>[2x]MLSPELLAKAFPFHFAF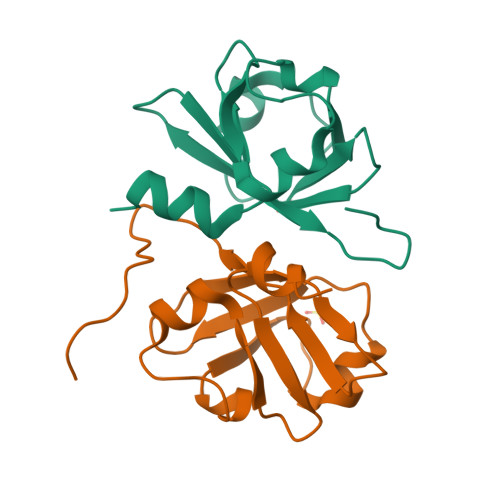SRNREIVQTGEVLERISPEPLVGKLIEQHFQINRPKILIDFDAISKQPRALFILEFLHNGMQLKGQMMYQPEEEVIFFLGSPWITDTTSLAPLGIKLK> MISNFRKFHGNKNQEKFNENLILNKENESILNYLD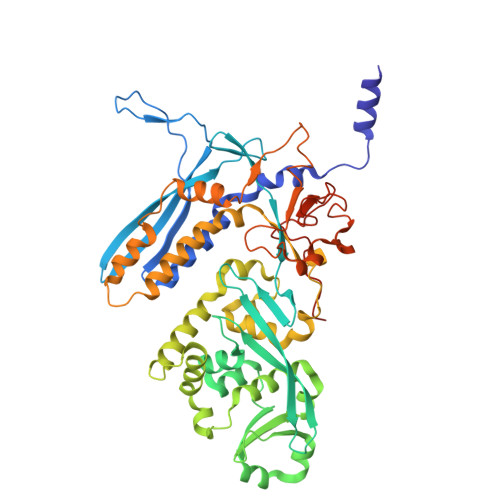PICKTLEIIPEITYLGSSVEPINKVYKFNKEEKTSDIERSELQLIKMSFLIEKDDKKEEINKFIYFPKLIDSQYFIINGNRYYPIYQLLDSGTYRTNKALTLKTLLMPIVLREKKETFDDINGETHTMLNVDLDLFKSKVPFLIYFFSKFGFEGTLEYFGLQDLIHVLMKEDLDQLDEDEINDNVIFMITKNISLVVDKNFFSNKNNQIIIATLLNCFNTRIKIDKIYEKDYWVKKLGGYFTTNNSNKQEKGEGIILSFERILDEWTKKILRTEEKNKEDIYSVVRWMINNYLALVKQDNMNLANKRIRLYEYLLHPLLIKFSKGTYRVLNNRNSNKFEKIKTIFSNIQEGFLVKKIINNELLRYDNSVNSISLFTLILRYTQSGPQSPFSSNSTNNKLRGLHPSYLGRLGLTSTSAGDPGASGSLTPFLELPENSYMHFTEEPEINLNIDDISIDEVIES> QGRAILTDRYINRGTAFTMEERQKLHILGRLPPVVETLEEQVARVYGQVKKYEKPINRYQHLVSVHSTNTTLYYATILAHLEEMLPIIYTPTVGEACMEYSHLFFRERGVYFNRLYKGQFRNIMRDAGYQKVEVVVITDGSRILGLGDLGSNGIGISIGKCSLYVAGAGIDPRLIVPVILDVGTNNERYLQDKDYLGMREKRLGDEEFYELLDEFMEAASAEWPNAVIQFEDFSNNHCFDIMERYQKKYRCFNDDIQGTGAVIAAGFLNAIKLSGVSPLQQRIVVFGAGSAAVGVANNIAALAARMYKFPVQDLVKTFYLVDTKGLVTTTRGDQLAAHKKLLARTDVSAEDSAKLRTLEEIVRFVKPTTLLGLGGVGPAFTEEIVKMVMQNTERPIIFPLSNPTSKAEVTPENAYKWTNGAAIVASGSPFPPTTIGGKTFKPSQGNNLYVFPGVGLGCALAQPTHIPEELLLTASESLNLLTTEGDLREGRLYPPLEDIHNISANVATDVILEAQRMKIDNN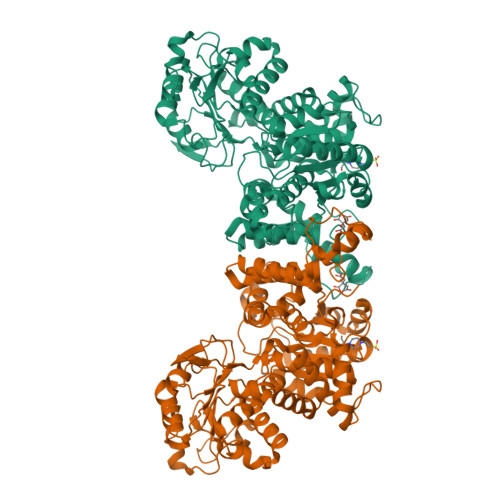KKLPRTRDELLAFVKKAMWKPVYSGEVGEQVL> MGSAIQDYFVKNRVGHSKPWESGKFKAADNFPDLSKHNNVMASQLTKELYEKYWDKVTPNGVTFDKCIQTGVDNPGNKFYGKKTGCVFGDEYSYECYKEFFDKCIEEIHHFKPSDKHPAPDLDHNKLVGGVFEDKYVKSCRIRCGRSVKGVCLPPAMSRAERRLVEKVVSDALGGLKGDLAGKYYPLTTMNEKDQEQLIEDHFLFEKPTGALLTTSGCARDWPDGRGIWHNNEKNFLVWINEEDHIRVISMQKGGDLKAVFSRFARGLLEVERLMKECGHGLMHNDRLGYICTCPTNMGTVVRASVHLRLAFLEKHPRFDEMLGKLRLGKRGTGG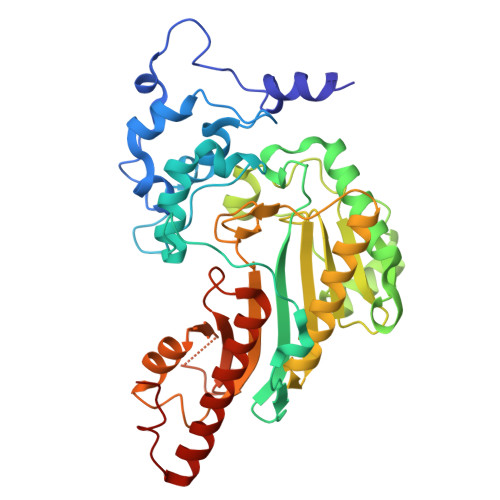ESSLATDSTYDISNWARLGKSERELVQVLVDGVNLLIACDKKLEAGQSIDDMIPK>[2x]GELMPPQLQNGLNLSAKVVQGSLDSLPQAVREFLENNAELCQPDHIHICDG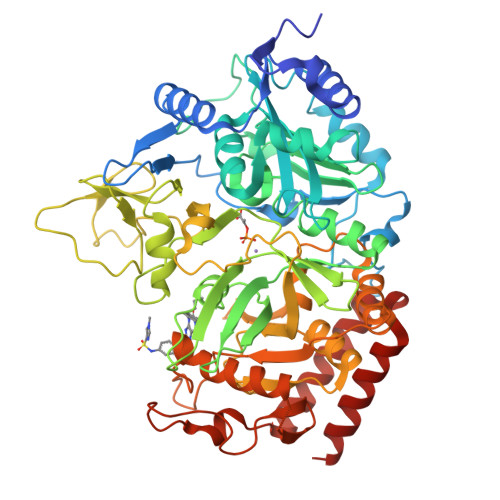SEEENGRLLGQMEEEGILRRLKKYDNCWLALTDPRDVARIESKTVIVTQEQRDTVPIPKTGLSQLGRWMSEEDFEKAFNARFPGCMKGRTMYVIPFSMGPLGSPLSKIGIELTDSPYVVASMRIMTRMGTPVLEALGDGEFVKCLHSVGCPLPLQKPLVNNWPCNPELTLIAHLPDRREIISFGSGYGGNSLLGKKCFALRMASRLAKEEGWLAEHMLVLGITNPEGEKKYLAAAFPSACGKTNLAMMNPSLPGWKVECVGDDIAWMKFDAQGHLRAINPENGFFGVAPGTSVKTNPNAIKTIQKNTIFTNVAETSDGGVYWEGIDEPLASGVTITSWKNKEWSSEDGEPCAHPNSRFCTPASQCPIIDAAWESPEGVPIEGIIFGGRRPAGVPLVYEALSWQHGVFVGAAMRSEATAAAEHKGKIIMHDPFAMRPFFGYNFGKYLAHWLSMAQHPAAKLPKIFHVNWFRKDKEGKFLWPGFGENSRVLEWMFNRIDGKASTKLTPIGYIPKEDALNLKGLGHINMMELFSISKEFWDKEVEDIEKYLVDQVNADLPCEIEREILALKQRISQM>MTLNTIALQLVPPNSDGPDGGREQAVEDARKVLRCAAETGLAGRIGHVMIPGMIEEDPDRPIPMKPKMDVLDFWTIIRPELPGIRGLCTQVTAFLDEPALRRRLGDLSAAGFDGIAFVGVPRTMNDGEGHGVAPTDALSMFADLVPNRGAILIPTRDGEQGRFEFKCERGATYGMTQLLYSDAIVGFLREFARRTDHRPEILLSFGFVPKLEAKVGLINWLIQDPGNPAVAAEQEFVRRLAGLEPADKRKLMVDLYKRVIDGVADLGFPLSVHLEATYGVSVPAFETFAEMLAYWSPGQG[2x]

Methylene‐tetrahydropterin reductases catalyze the reduction of a methylene to a methyl group bound to a reduced pterin as C1 carrier in various one‐carbon (C1) metabolisms. F420‐dependent methylene‐tetrahydromethanopterin (methylene‐H4MPT) reductase (Mer) and the flavin‐independent methylene‐tetrahydrofolate (methylene‐H4F) reductase (Mfr) use a ternary complex mechanism for the direct transfer of a hydride from F420H2 and NAD(P)H to the respective methylene group, whereas FAD‐dependent methylene‐H4F reductase (MTHFR) uses FAD as prosthetic group and a ping–pong mechanism to catalyze the reduction of methylene‐H4F. Mutational analysis of four functional amino acids, which are similarly positioned in the three reductase structures, indicated despite the insignificant sequence identity, a common catalytic mechanism with a 5‐iminium cation of methylene‐tetrahydropterin as intermediate protonated by a shared glutamate. Based on mutational and kinetic analysis, evidence has been provided that all three methylene‐tetrahydropterin reductases have the same fold, similar methylene‐tetrahydropterin binding positions, and the same basic catalytic mechanism; however, the binding modes of the C1 carriers and reductants significantly deviate.

The flavin‐independent enzymes, named Mfr (Gehl et al., 2023), was currently identified only in mycobacteria as a monomeric enzyme. Recently, we reported the crystal structure of Mfr from Mycolicibacterium hassiacum (hMfr) and provided evidence that Glu9 in the active site is the key catalytic residue for 5‐iminium cation formation. Thus, the mechanism of eMTHFR and hMfr is basically identical. Position A contains a glutamate residue in all three reductases. In hMfr and jMer, apparent k cat of the equivalent Glu9Gln and Glu6Gln variants decreased from 594 to 1.3 min−1 (0.2%) (Gehl et al., 2023), and from 18,200 to 71 min−1 (0.4%), respectively. Neither variant showed a significant increase in the apparent K m for their respective C1 carrier, suggesting that glutamate and glutamine bind in a related manner. In addition, we obtained the crystal structures of the inactive variants jMer_E6Q, and hMfr_E9Q to exclude perturbations of the active sites. X‐ray structure analysis of the jMer_E6Q and hMfr_E9Q variants were performed and the structures were compared with the wild‐type enzyme, which confirmed unchanged active site architectures compared with the wild‐type enzymes.> MEDKGKTFFGQPLGLSTLFMTEMWERFSYYGMRAILLYYMWFLISTGDLHITRATAASIMAIYASMVYLSGTIGGFV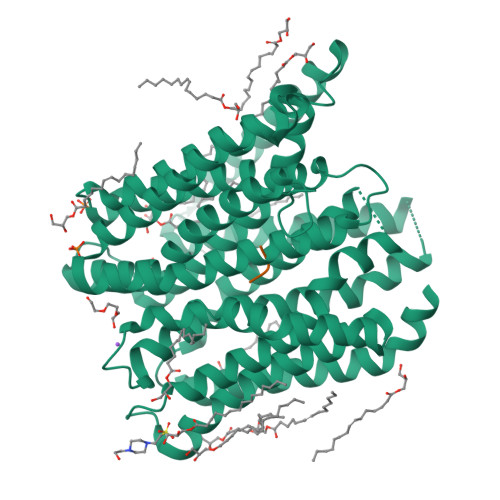ADRIIGARPAVFWGGVLIMLGHIVLALPFGASALFGSIILIIIGTGFLKPNVSTLVGTLYDEHDRRRDAGFSIFVFGINLGAFIAPLIVGAAQEAAGYHVAFSLAAIGMFIGLLVYYFGGKKTLDPHYLRPTDPLAPEEVKPLLVKVSLAVAGFIAIIVVMNLVGWNSLPAYINLLTIVAIAIPVFYFAWMISSVKVTSTEHLRVVSYIPLFIAAVLFWAIEEQGSVVLATFAAERVDSSWFPVSWFQSLNPLFIMLYTPFFAWLWTAWKKNQPSSPTKFAVGLMFAGLSFLLMAIPGALYGTSGKVSPLWLVGSWALVILGEMLISPVGLSVTTKLAPKAFNSQMMSMWFLSSSVGSALNAQLVTLYNAKSEVAYFSYFGLGSVVLGIVLVFLSKRIQGLMQGVE;> FAQ> GSWFFGKIPRAKAEEMLSKQRHDGAFLIRESESAPGDFSLSVKFGNDVQHFKVLRDGAGKYFLWVVKF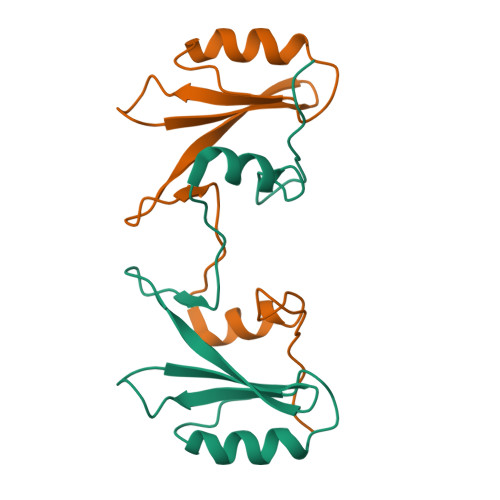NSLNELVDYHRSTSVSRNQQIFLRDIE> LDSGRFSRKQLDKKYKHAGDFGISDTKKNRETLTKFRDAIEEHLSDKDTVEKGTYRREKGSKVYFNP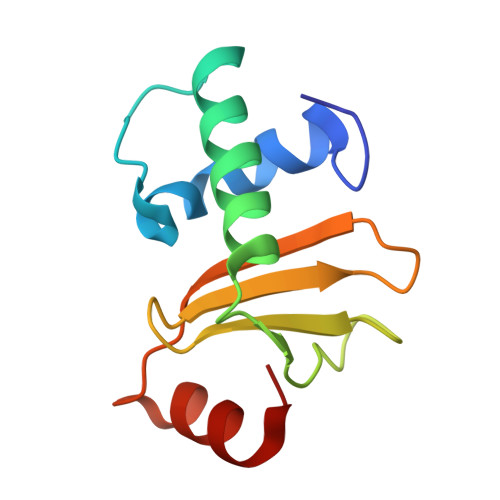NTMNVVIIKSNGEFLSGWKINPDADNGRIYLETGEL>[3x]XGPPGPPGPPGPPGKLGPPGPP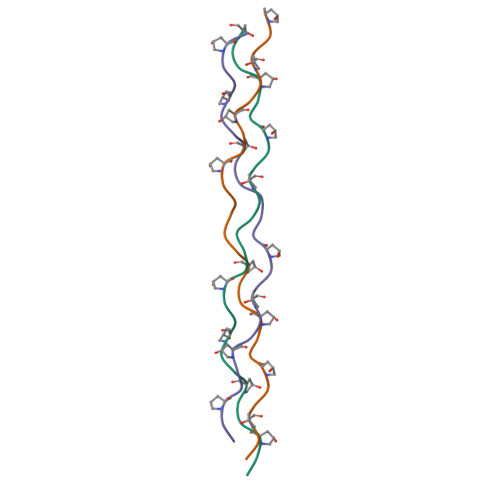GPPGPPX>[2x]MDAELKIFVSSQHQPDIWRKALDQYEAKTPGVKVVIETGGNTSEMQAQYLNTVMSAKDSSLDVLMLDVIRPAQFATAGWTSDFSGKDLSAYLPTYAEANTVNGKIVALPAFADSMFLYYRKDLLDKYGIKPPTTWDELKEASKKVMEGEKNPELQGLSFQGKAIEGAVCTFLLPYWSEGKSLVENGKLNFDNKAAVDSLKLWKS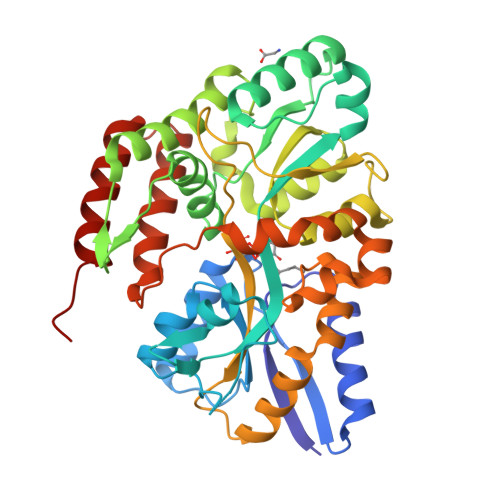FVDDGISKKNISEVATDDTRKEFQAGKVLFAVNWSYAWTHFQGKESQVNDKVGVARLPAVKGGEQTTCLGGWEFGVSAYSKQQDEAKKLVEYLSSQDVSKFMAINAALLPTYAALYKDADVTKTIPWFADALPVVETAKARPVTPRYNEVSETIRTTVNGVLAGVMTPEDGAKQMESRLRRVLRLEHHHHHH>MTAKLLHWAPFTIKTLTTKDIDNLKVEIKDFTGLNTKDKLSSDDAKQESQKAFDAINKIVDAFAENNKADIKDKKISDSTIAAANNLKTKADNALKFVNENASVTNWTDDR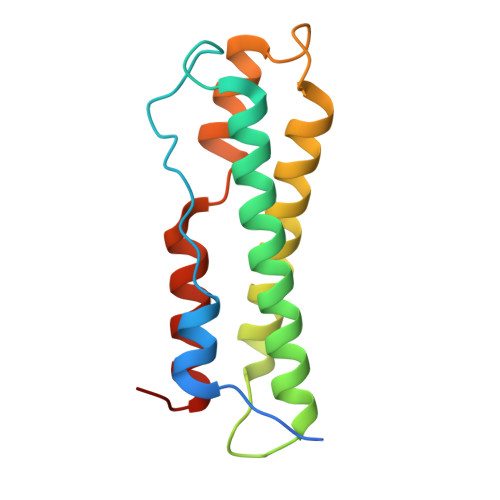VQDFVNNKVVKTKEINDLLSQAKTDLKLQS[2x]> MENAHTKTVEEVLGHFGVNESTGLSLEQVKKLKERWGSNELPAEEGKTLLELVIEQFEDLLVRILLLAACISFVLAWFEEGEETITAFVEPFVILLILVANAIVGVWQERNAENAIEALKEYEPEMGKVYRQDRKSVQRIKAKDIVPGDIVEIAVGDKVPADIRLTSIKSTTLRVDQSILTGESVSVIKHTDPVPDPRAVNQDKKNMLFSGTNIAAGKAMGVVVATGVNTEIGKIRDEMVATEQERTPLQQKLDEFGEQLSKVISLICIAVWIINIGHFNDPVHGGSWIRGAIYYFKIAVALAVAAIPEGLPAVITTCLALGTRRMAKKNAIVRSLPSVETLGCTSVICSDKTGTLTTNQMSVCRMFILDRVEGDTCSLNEFTITGSTYAPIGEVHKDDKPVNCHQYDGLVELATICALCNDSALDYNEAKGVYEKVGEATETALTCLVEKMNVFDTELKGLSKIERANACNSVIKQLMKKEFTLEFSRDRKSMSVYCTPNKPSRTSMSKMFVKGAPEGVIDRCTHIRVGSTKVPMTSGVKQKIMSVIREWGSGSDTLRCLALATHDNPLRREEMHLEDSANFIKYETNLTFVGCVGMLDPPRIEVASSVKLCRQAGIRVIMITGDNKGTAVAICRRIGIFGQDEDVTSKAFTGREFDELNPSAQRDACLNARCFARVEPSHKSKIVEFLQSFDEITAMTGDGVNDAPALKKAEIGIAMGSGTAVAKTASEMVLADDNFSTIVAAVEEGRAIYNNMKQFIRYLISSNVGEVVCIFLTAALGFPEALIPVQLLWVNLVTDGLPATALGFNPPDLDIMNKPPRNPKEPLISGWLFFRYLAIGCYVGAATVGAAAWWFIAADGGPRVSFYQLSHFLQCKEDNPDFEGVDCAIFESPYPMTMALS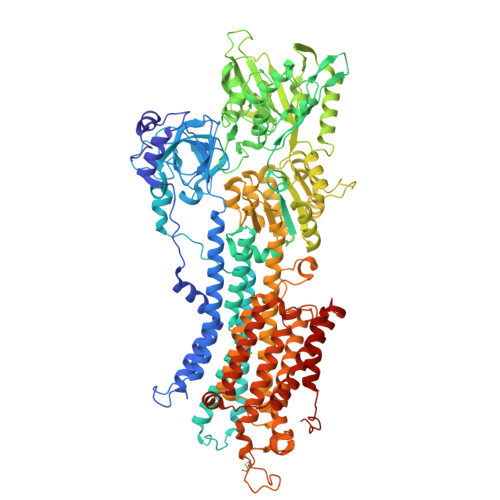VLVTIEMCNALNSLSENQSLLRMPPWENIWLVGSICLSMSLHFLILYVEPLPLIFQITPLNVTQWLMVLKISLPVILMDETLKFVARNYLEPGKECVQPATKSCSFSACTDGISWPFVLLIMPLVIWVYSTDTNFSDMFWS Nitric oxide (NO) is an important signaling molecule critical in the cardiovascular, neuronal, and immune systems. The enzyme responsible for generating NO is nitric oxide synthase (NOS), a P450-like heme thiolate enzyme that oxidizes l-arginine to NO and L-citrulline. Humans and other mammals express three different NOS isoforms: endothelial NOS (eNOS), neuronal NOS (nNOS), and inducible NOS (iNOS). nNOS is an important therapeutic target since the overproduction of NO by nNOS in the brain is associated with a number of neurodegenerative diseases. Thus, nNOS is an attractive target for therapeutic intervention. In our efforts to develop inhibitors selective for neuronal nitric oxide synthase (nNOS) over endothelial nitric oxide synthase (eNOS), we found that nNOS can undergo conformational changes in response to inhibitor binding that does not readily occur in eNOS. Here, we used a combination of crystallography, mutagenesis, and computational methods to better understand the structural basis for these differences in NOS inhibitor binding.

We asked the questions, how can the inhibitor displace BH4, and does the inhibitor displacing BH4 in hnNOS bind synergistically or independently from the inhibitor bound in the active site? To explore these questions, we “knocked out” the active site inhibitor binding by mutating the active site Glu to Gln in both hnNOS and heNOS to generate hnNOS E597Q and heNOS E361Q. 4 binds in neither the active site nor the BH4 site in these hnNOS and heNOS mutants. Most unexpected, however, was that the same backbone changes in the region of hnNOS residues 598–611 were observed when two molecules bind to wild-type hnNOS occurred in the compound 4-soaked hnNOS E597Q structure, even though no inhibitor was bound in the active site and BH4 remained bound in its site. Therefore, the simple elimination of one charge in the active site results in this structural change without the need for inhibitor binding. This result underscores the complex interplay between the active site and the region that undergoes the conformational change several Ångströms away. In addition, mutating the active site Glu to Gln in nNOS resulted in the same conformational change that results from two inhibitors binding. This suggests that when two inhibitors bind, the first one enters the active site and hydrogen bonds with the active site Glu, lowering the energetic barrier to the conformational change required to bind the second molecule that displaces BH4.

>[4x]CPRFLKVKNWETEVVLTDTLHLKSTLETGCTEYICMGSIMHPSQHARRPEDVATKDQLFPLAKEFIDQYYSSIKRFGSKAHMERLEEVNKEIDTTSTYQLKDTELIYGAKHAWRNASRCVGRIQWSKLQVFDARDCTTAHGMFNYICNHVKYATNKGNLRSAITIFPQRTDGKHDFRVWNSQLIRYAGYKQPDGSTLGDPANVQFTEICIQQGWKPPRGRFDVLPLLLQANGNDPELFQIPPELVLEVPIRHPKFEWFKDLGLKWYGLPAVSNMLLEIGGLEFSACPFSGWYMGTQIGVRDYCDNSRYNILEEVAKKMNLDMRKTSSLWKDQALVEINIAVLYSFQSDKVTIVDHHSATESFIKHMENEYRCRGGCPADWVWIVPPMSGSITPVFHQEMLNYRLTPSFEYQPDPWNTHVWKLV>[2x]GKLEARAALNQALEMKR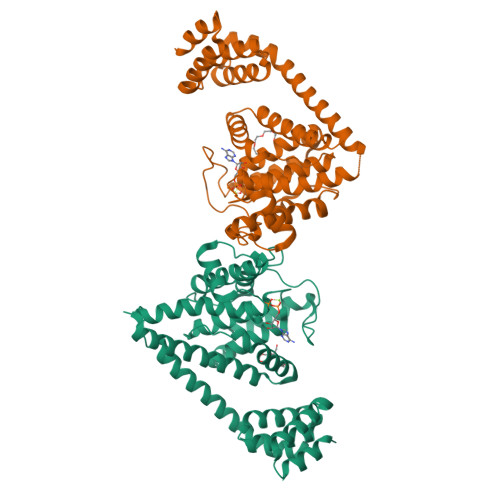QGKREKAQKLFMHALKMDPDFVDALTEFGIFSEEDKDIIQADYLYTRALTISPYHEKALVNRDRTLPLVEEIDQRYFSIIDSKVKKVMSIPKGNSALRRVMEETYYHHIYHTVAIEGNTLTLSEIRHILETRYAVPGKSLEEQNEVIGMHAAMKYINTTLVSRIGSVTISDVLEIHRRVLGYVDPVEAGRFRTTQVLVGHHIPPHPQDVEKQMQEFVQWLNSEEAMNLHPVEFAALAHYKLVYIHPFIDGNGRTSRLLMNLILMQAGYPPITIRKEQRSDYYHVLEAANEGDVRPFIRFIAKCTETTLDTLLFATTEYSVALPEAQP> MVSRYVPDMGDLIWVDFDPTKGSAQAGHRPAVVLSPFMYNNKTGMCLCVPCTTQSKGYPFEVVLSGQERDGVALADQVKSIAWRARGATKKGTVAPEELQLIKAKINVLIG;> XSHLFWAQFDEYFX

The toxin MazF is an endoribonuclease that recognizes ACA subsequences within single-stranded mRNAs and rRNA precursors, and catalyzes the hydrolysis of adjacent phosphodiester bonds. , In turn, the antitoxin MazE prevents MazF catalysis by the formation of a protein–protein complex that blocks the access of substrates to the toxin active site. Each monomer is composed of seven β-strands forming an antiparallel and highly twisted β-sheet, followed by a long C-terminal α-helix. The toxin displays a large concave cavity at the homodimer interface, whose central region is characterized by a positive surface electrostatic potential, while the edges are amphiphilic with positively charged and hydrophobic residues. The N-acetylated and C-amidated synthetic peptide, named Small Antitoxin of MazF (SamF), interacts specifically and with high affinity with MazF, preventing its ribonucleolytic activity by competing with RNA substrates for the same binding site.

Therefore, all biophysical experiments, with the sole exception of MazF kinetic assays, were carried out with the catalytically less active mutant containing glutamic acid 24 replaced with alanine (MazFE24A), which resembles the WT protein structure and leads to homogeneous samples that are produced at high yields in E. coli. Structural deviations are mainly seen in the β-strands S3, S4, and S5 that are slightly shorter in the peptide-bound state, which causes an elongation in the corresponding interstrand loops. As in the unbound state, SamF adopts a helical conformation when it is complexed with MazFE24A. Two molecules of SamF bind at the dimeric interface of MazFE24A, where they form intermolecular contacts with residues in α-helix H1 of one subunit and with residues in α-helix H3 as well as in the interstrand loops S3–S4 of the opposite subunit. The binding site of SamF is the same one that accommodates MazE subsequence 54–67 in the MazE-MazF complex. The aromatic ring of SamF’s F4 is buried into a hydrophobic pocket, in which it gets close to the side chains of V108 at the α-helix H3 and P59/F60 at the interstrand loops S3–S4 of the same monomer. The side chain of SamF’s F8 is sandwiched between the aromatic rings of F60/Y39 and the aliphatic side chains of M38 and P59, indicating that this residue may have a central role in toxin binding. At the α-helix H1 of MazFE24A, the side chain of K42 is in a favorable orientation to form a salt bridge with SamF’s D9. As SamF, the substrate makes pronounced interactions with α-helix H1 and the interstrand loop S3–S4 of the toxin, and thus, upon binding, SamF blocks the access to the toxin substrate binding site, a similar inhibition mechanism that should be employed by the MazE_54–67 polypeptide region.>MSVAYNPQTKQFHLRAGKASYVMQLFRSGYLAHVYWGKAVRDVRGARAFPRLDRAFSPNPDPSDRTFSLDTLLQEYPAYGNTDFRAPAYQVQLENGSTVTDLRYKTHRIYKGKPRLNGLPATYVEHEQEAETLEIVLGDALIGLEVTLQYTAYEKWNVITRSARFENKGGERLKLLRALSMSVDFPTADYDWIHLPGAWGRERWIERRPLVTGVQAAESRRGASSHQQNPFIALVAKNADEHQGEVYGFSFVYSGNFLAQIEVDQFGTARVSMGINPFDFTWLLQPGESFQTPEVVMVYSDQGLNGMSQTYHELYRTRLARGAFRDRERPILINNWEATYFDFNEEKIVNIARTEAELGIELVVLDDGWFGERDDDRRSLGDWIVNRRKLPNGLDGLAKQVNELGLQFGLWVEPEMVSPNSELYRKHPDWCLHVPNRPRSEGRNQLVLDYSREDVCDYIIETISNVLASAPITYVKWAMNRHMTEIGSSALPPERQRETAHRYMLGLYRVMDEITSRFPHILFESCSGGGGRFDPGMLYYMPQTWTSDNTDAVSRLKIQYGTSLVYPIS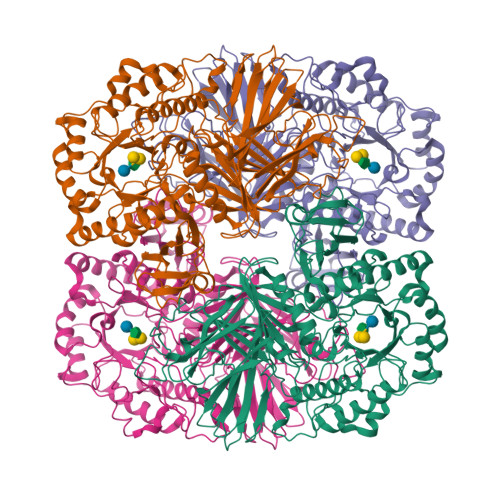AMGAHVSAVPNHQVGRVASLKTRGHVAMSGNFGYELDITKLTETEKQMMKQQVAFYKDVRRLVQFGTFYRLLSPFEGNEAAWMFVSADRSEALVAYFRVLAEANAPLSYLRLKGLDSNQDYEIEGLGVYGGDELMYAGVALPYRSSDFISMMWRLKAVQQ[4x]> MADMADMTIKEGFAPFGDYQTWYRITGDLRGGGTPLVILHGGPGCTHDYVDSFKDIANTGRAVIHYDQLGNGKSTHLPDMGSEFWTVDLFLSELDNLLEYLEIADDYALLGQSWGGMLASEHAVLQPTGLQALIIANSPADMHTWVSEANRLREELPDDVQATLLKHEEAGTLTDPAYLTASRVFYDRHVCRITPWPVEVERTFHQIDEDPTVYRAMNGPTEFHVIGTMKDWSIVD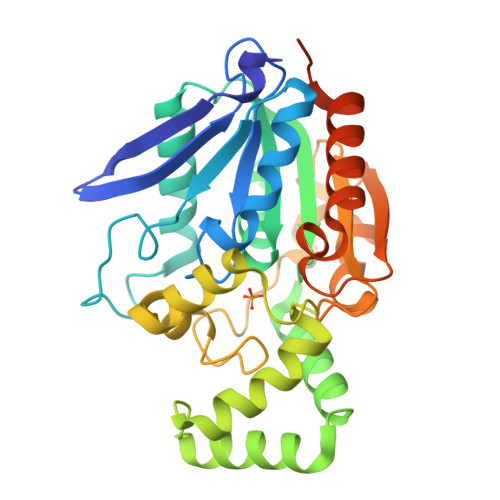RLSNINVPTLVISGFYDEATPLVIQPYVDNIPDVRQSVFQESSHMPHVEERMACMGRVADFLDEVATSGKALPGVKARFGIEGRLEHHHHHH>ALYEDPPDQKTSPSGKPATLKICSWNVDGLRAWIKKKGLDWVKEEAPDILCLQETKCSE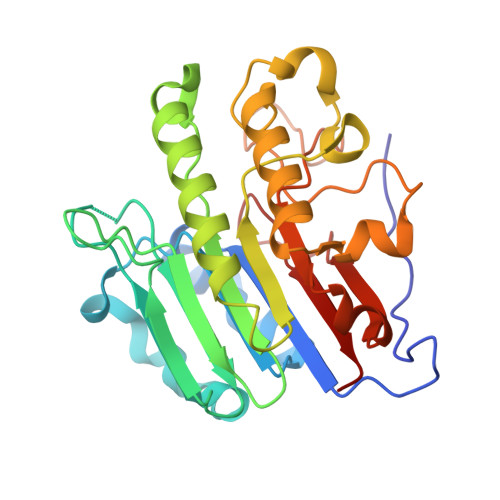NKLPAELQELPGLSHQYWSAPSDKEGYSGVGLLSRQAPLKVSYGIGDEEHDQEGRVIVAEFDSFVLVTAYVPNAGRGLVRLEYRQRWDEAFRKFLKGLASRKPLVLCGDLNVAHEEIDLRNPKGNKKNAGFTPQERQGFGELLQAVPLADSFRHLYPNTPYAYTFWTYMMNARSKNVGWRLDYFLLSHSLLPALCDSKIRSKALGSDHCPITLYLAL[2x]>[4x]MEEPEEPADSGQSLVPVYIYSPEYVSM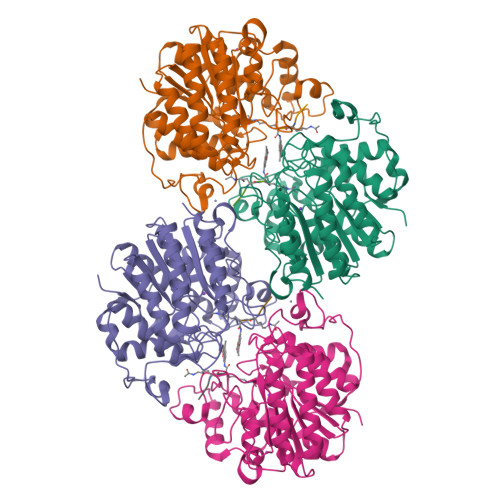CDSLAKIPKRASMVHSLIEAYALHKQMRIVKPKVASMEEMATFHTDAYLQHLQKVSQEGDDDHPDSIEYGLGYDCPATEGIFDYAAAIGGATITAAQCLIDGMCKVAINWSGGWHAAKKDEASGFCYLNDAVLGILRLRRKFERILYVDLDLHHGDGVEDAFSFTSKVMTVSLHKFSPGFFPGTGDVSDVGLGKGRYYSVNVPIQDGIQDEKYYQICESVLKEVYQAFNPKAVVLQLGADTIAGDPMCSFNMTPVGIGKCLKYILQWQLATLILGGGGYNLANTARCWTYLTGVILGKTLSSEIPDHEFFTAYGPDYVLEITPSCRPDRNEPHRIQQILNYIKGNLKHVVIEGRSHHHHHH;>XRHKK[4x]>MSSGLYLYGIFPDPIPETVTLQGLDSQLVYSQIIDGFTFLYSEAKQEKYLASRRNLISHEKVLEQAMHAGFRTLLPLRFGLVVKNWETVVTQLLQPYKAQLRELFQKLAGRREVSVKIFWDSKAELQAMMDSHQDLKQKRDQMEGKALSMEEVIHIGQLIESNLLSRKESIIQVFFDELKPLADEVIESDPMTEDMIYNAAFLIPWENESIFSQQVESIDHKFDERLRIRYNNFTAPYTFAQISHHHHHH[2x]

Gas vesicles (GVs), a unique class of intracellular bubble-like nanostructures, are found in many aquatic and soil microbes including halophilic archaea, photosynthetic bacteria, and heterotrophic bacteria. As previously reported, formation of GVs is related to a conserved cluster of 8 ~ 14 genes (termed gas vesicle protein gene cluster, or gvp gene cluster for short), encoding two major structural proteins and several essential minor components that might putatively function as chaperones, nucleators and regulators. In addition, GvpF is reported to be a structural protein localized at the inner surface of GVs. Here we found that Anabaena sp. PCC 7120 possesses an intact gvp gene cluster, which shares an organization similar to that of previously identified GV-forming cyanobacteria.

To further investigate the putative GVs of Anabaena sp. PCC 7120 from the structural point of view, all Gvp proteins, except for GvpA and GvpC, were successfully overexpressed, purified and applied to crystal screening; however, only the crystal structure of GvpF was eventually solved at 2.55 Å resolution in the space group C2221. Anabaena sp. PCC 7120 GvpF is composed of two structurally separated domains, both of which display a fold in α + β class, followed by a C-terminal tail inserted into the middle area of the two domains. Further structural analysis showed that the N-domain of GvpF displays an architecture in which a six-stranded β-sheet (β1-β6) is sandwiched by two α-helices (α1-α2) and the helix η1, whereas the C-domain adopts a modified ferredoxin fold owing to an extension region consisting of three consecutive helices (α4, α5 and the N-terminal segment of α6). Moreover, the additional C-terminal tail provides an interface for the N-domain and C-domain to pack against each other, resulting in the structural stability and correct folding of GvpF. Superposition of the two structures showed a very similar structure, except that GvpF of Anabaena sp. PCC 7120 possesses a shorter helix α5 in the C-domain. Besides, structure-based multiple-sequence alignment revealed that GvpF proteins are highly conserved among diverse species of cyanobacteria. It indicated that Anabaena sp. PCC 7120 GvpF might also function as a structural protein involved in forming GVs as that of M. aeruginosa PCC 7806. Moreover, structural combined with enzymatic investigations suggested that GvpF and GvpN are structurally and enzymatically conserved, respectively.A key component of the LDAC is the evolutionarily conserved ER membrane protein seipin. Seipin consists of an evolutionarily conserved ER-lumenal domain and flanking transmembrane (TM) segments, and less conserved cytoplasmic N- and C-terminal regions with lengths that vary among species. Lipid droplets (LDs) form in the endoplasmic reticulum by phase separation of neutral lipids. This process is facilitated by the seipin protein complex, which consists of a ring of seipin monomers, with a yet unclear function.

As an alternative, we purified the yeast seipin Sei1–Ldb16 complex by affinity and size-exclusion chromatography from a strain that overproduced both proteins from the GAL1 promoter at their endogenous loci. We refined the class with the highest predicted resolution with C5 symmetry, which revealed a roughly 145-Å diameter complex with two alternating conformations of the TM segments that were invisible in the three-dimensional (3D) reconstruction with C10 symmetry. We designated these alternate conformations A and B. In this map, nearly all of the lumenal domain of seipin and most of the TM regions are well resolved with an overall resolution of roughly 3.2 Å. Our model for yeast seipin revealed a decameric complex with the shape of a domed cage, with the lumenal domains forming the floor of the cage, predicted to sit beneath the lumenal leaflet of the ER membrane. The TM segments form the side walls of the cage and are tilted toward the center of the oligomer, coming together in a dome-shape at the cytoplasmic side of the complex. Two ‘switch’ regions (residues 40–55 and 231–243), representing the biggest differences between conformations A and B, connect the ring of folded lumenal domains to the TM segments of seipin. In conformation A, the N-terminal TM helix is tilted roughly 40° toward the center of the oligomer, whereas the C-terminal switch region adopts a kinked α-helix connected to the second TM helix. In conformation B, the C-terminal TM helix exhibits a continuously extended helix through the switch region and lacks the kink found in conformation A. As a result, the N-terminal TM helix in conformation B is tilted further (roughly 60°) toward the center of the oligomeric assembly and both TM segments lie close to the N-terminal TM helix of the neighboring conformation A monomer. The fly and human lumenal domains possess a longer central helix that is hydrophobic, interacts with LDAF1 in humans, inserts into the ER bilayer and is implicated in binding TGs in molecular dynamics simulations. In contrast, yeast seipin has two short helices with several charged residues (for example, Q169, E172, Q173, E184) and a different orientation compared with human or fly seipin, which likely does not insert into the membrane.

>[10x]MKINVSRPLQFLQWSSYIVVAFLIQLLIILPLSILIYHDFYLRLLPADSSNVVPLNTFNILNGVQFGTKFFQSIKSIPVGTDLPQTIDNGLSQLIPMRDNMEYKLDLNLQLYCQSKTDHLNLDNLLIDVYRGPGPLLGAPGGSNSKDEKIFHTSRPIVCLALTDSMSPQEIEQLGPSRLDVYDEEWLNTIRIEDKISLESSYETISVFLKTEIAQRNLIIHPESGIKFRMNFEQGLRNLMLRKRFLSYIIGISIFHCIICVLFFITGCTAFIFVRKGQEKSKKHS In this work, we exhaustively probe the ability of all 36 immobile HJ sequences to form DNA crystals in two different designed systems. Three separate self-assembling DNA crystal systems are described in this report: the “4 × 5” and “4 × 6” designs (collectively referred to as the 4 × N systems), and a third construct with a “scrambled” sequence variant of the 4 × 6 lattices. Self-assembly was mediated by three constituent oligonucleotides: (S1) containing four sequence repeats of either 5 or 6 bases; (S2) composed of 21 bases containing complementary regions to both (S1); and (S3) which forms the second junction crossover. The HJ serves as the fundamental component at the core of each unit, and the ultimate assembly of the full lattice is facilitated by the complementary 2-base sticky ends that tail each duplex.

Because the 4 × 6 system yielded R3 symmetry in 5 of 17 junctions, we considered whether the downstream sequences adjacent to the junction could play a role in crystallization efficiency, junction angle, and symmetry preference, or if the HJ alone was the singular determinant. To investigate this possibility, we designed “scrambled” sequences with targeted base substitutions, while maintaining GC content, along each “stem”. Contrary to the buffer preference observed with the native P32 crystals, the scrambled systems exhibited an exclusive preference towards low salt buffers, much like the native R3 crystals. Remarkably, only J1 and J2 retained the P32 symmetry, with all others yielding an R3 lattice. There appeared to be only a marginal difference in the average cell lengths in the R3 scramble crystals (a = b = 113.04 c = 51.10) relative to the native 4 × 6 sequences: the a, b axis trended ~2 Å shorter and c ~1.3 Å longer, whereas in the J1 and J2 cases, the crystals were in good agreement with the original 4 × 6 motif. The average angles of the R3 and P32 crystals were 61.00° (σ = 1.21) and 58.05° (σ = 1.39), respectively. Further, we observed modest improvements in resolution, reaching as high as 2.7 Å in J36. Notably, all junctions preventing crystallization compared to its original counterpart remained fatal and all relative cavity dimensions and volumes remained unperturbed. However, in the majority of the crystal structures reported here, the cacodylate anion indeed fits best into the electron density map of our X-ray structures, due to the presence of sodium cacodylate in the crystallization solution.

> GCGTCA;> GAACGACAGTGACGCCGACTC;> TCGAGTCG;> CTGTCGT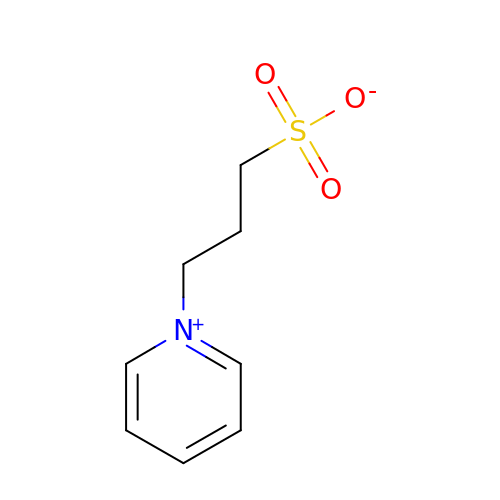3-PYRIDINIUM-1-YLPROPANE-1-SULFONATE | C8 H11 N O3 S | REEBJQTUIJTGAL-UHFFFAOYSA-N> TVPASVDWRKKGAVTSVKDQGQCGSCWAFSTIVAVEGINQIKTNKLVSLSEQELVDCDTDQNQGCNGGLMDYAFEFIKQRGGITTEANYPYEAYDGTCDVSKENAPAVSIDGHENVPENDENALLKAVANQPVSVAIDAGGSDFQFYSEGVFTGSCGTELDHGVAIVGYGTTIDGTKYWTVKNSWGPEWGEKGYIRMERGISDKEGLCGIAMEA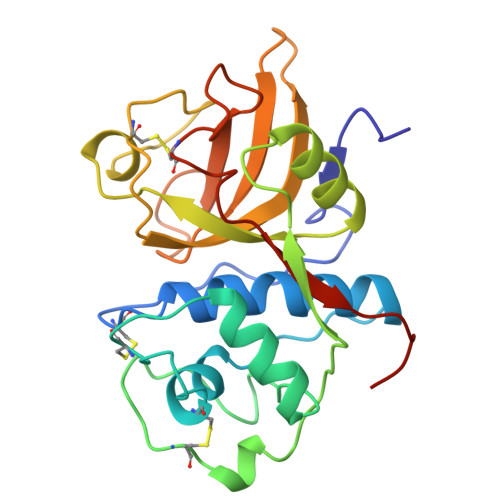SYPIKKSSNNPSGIK> SGSGSSPELDELWKRVKKLVTELLEQAERAGDPEEIFKLLEVAAALVFLAEMFLRLAAIQEKATDPEIQELAERVLRLIKRLLEEAERAGDPRRIRELVEVASQL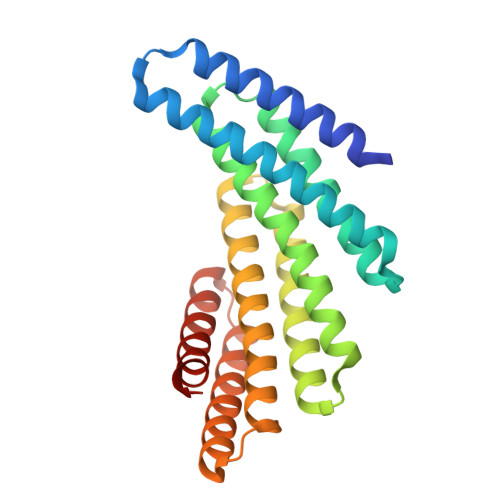AFLLELFYRLKEIQERATDPEIQELAERVLRLIKKLLKAAEEAGDPRKIHKLVFVAIVLLFLLQTFYRLKEIQEKATDPEIQRKAQEVLEKIKRLLEAAERAGDPAKILLYVIRALLLAMELKFAYRKR> GMSDVAETLDPLRLPLQGERLIEASAGTGKTFTIAALYLRLLLGLGGSAAFPRPLTVEELLVVTFTEAATAELRGRIRSNIHELRIACLRETTDNPLYERLLEEIDDKAQAAQWLLLAERQMDEAAVFTIHGFCQRMLNLNAFESGMLFEQQLIEDESLLRYQACADFWRRHCYPLPREIAQVVFETWKGPQALLRDINRYLQGEAPVIKAPPPDDETLASRHAQIVARIDTVKQQWRDAVGELDALIESSGIDRRKFNRSNQAKWIDKISAWAEEETNSYQLPESLEKFSQRFLEDRTKAGGETPRHPLFEAIDQLLAEPLSIRDLVITRALAEIRETVAREKRRRGELGFDDMLSRLDSALRSESGEVLAAAIRTRFPVAMIDEFQDTDPQQYRIFRRIWHHQPETALLLIGDPKQAIYAFRGADIFTYMKARSEVHAHYTLDTNWRSAPGMVNSVNKLFSQTDDAFMFREIPFIPVKSAGKNQALRFVFKGETQPAMKMWLMEGESCGVGDYQSTMAQVCAAQIRDWLQAGQRGEALLMNGDDARPVRASDISVLVRSRQEAAQVRDALTLLEIPSVYLSNRDSVFETLEAQEMLWLLQAVMTPERENTLRSALATSMMGLNALDIETLNNDEHAWDVVVEEFDGYRQIWRKRGVMPMLRALMSARNIAENLLATAGGERRLTDILHISELLQEAGTQLESEHALVRWLSQHILEPDSNASSQQMRLESDKHLVQIVTIHKSKGLEYPLVWLPFITNFRVQEQAFYHDRHSFEAVLDLNAAPESVDLAEAERLAEDLRLLYVALTRSVWHCSLGVAPLVRRRGDKKGDTDVHQSALGRLLQKGEPQDAAGLRTCIEALCDDDIAWQTAQTGDNQPWQVNDVSTAELNAKTLQRLPGDNWRVTSYSGLQQRXXXXXXXXXXXXXXXXXXXXXXXXXPTLTPHQFPRGASPGTFLHSLFEDLDFTQPVDPNWVREKLELGGFESQWEPVLTEWITAVLQAPLNETGVSLSQLSARNKQVEMEFYLPISEPLIASQLDTLIRQFDPLSAGCPPLEFMQVRGMLKGFIDLVFRHEGRYYLLAYKSNWLGEDSSAYTQQAMAAAMQAHRYDLQYQLYTLALHRYLRHRIADYDYEHHFGGVIYLFLRGVDKEHPQQGIYTTRPNAGLIALMDEMFAGMTLEEA;> MLRVYHSNRLDVLEALMEFIVERERLDDPFEPEMILVQSTGMAQWLQMTLSQKFGIAANIDFPLPASFIWDMFVRVLPEIPKESAFNKQSMSWKLMTLLPQLLEREDFTLLRHYLTDDSDKRKLFQLSSKAADLFDQYLVYRPDWLAQWETGHLVEGLGEAQAWQAPLWKALVEYTHQLGQPRWHRANLYQRFIETLESATTCPPGLPSRVFICGISALPPVYLQALQALGKHIEIHLLFTNPCRYYWGDIKDPAYLAKLLTRQRRHSFEDRELPLFRDSENAGQLFNSDGEQDVGNPLLASWGKLGRDYIYLLSDLESSQELDAFVDVTPDNLLHNIQSDILELENRAVAGVNIEEFSRSDNKRPLDPLDSSITFHVCHSPQREVEVLHDRLLAMLEEDPTLTPRDIIVMVADIDSYSPFIQAVFGSAPADRYLPYAISDRRARQSHPVLEAFISLLSLPDSRFVSEDVLALLDVPVLAARFDITEEGLRYLRQWVNESGIRWGIDDDNVRELELPATGQHTWRFGLTRMLLGYAMESAQGEWQSVLPYDESSGLIAELVGHLASLLMQLNIWRRGLAQERPLEEWLPVCRDMLNAFFLPDAETEAAMTLIEQQWQAIIAEGLGAQYGDAVPLSLLRDELAQRLDQERISQRFLAGPVNICTLMPMRSIPFKVVCLLGMNDGVYPRQLAPLGFDLMSQKPKRGDRSRRDDDRYLFLEALISAQQKLYISYIGRSIQDNSERFPSVLVQELIDYIGQSHYLPGDEALNCDESEARVKAHLTCLHTRMPFDPQNYQPGERQSYAREWLPAASQAGKAHSEFVQPLPFTLPETVPLETLQRFWAHPVRAFFQMRLQVNFRTEDSEIPDTEPFILEGLSRYQINQQLLNALVEQDDAERLFRRFRAAGDLPYGAFGEIFWETQCQEMQQLADRVIACRQPGQSMEIDLACNGVQITGWLPQVQPDGLLRWRPSLLSVAQGMQLWLEHLVYCASGGNGESRLFLRKDGEWRFPPLAAEQALHYLSQLIEGYREGMSAPLLVLPESGGAWLKTCYDAQNDAMLDDDSTLQKARTKFLQAYEGNMMVRGEGDDIWYQRLWRQLTPETMEAIVEQSQRFLLPLFRFNQS;> MGKLQKQLLEAVEHKQLRPLDVQFALTVAGDEHPAVTLAAALLSHDAGEGHVCLPLSRLENNEASHPLLATCVSEIGELQNWEECLLASQAVSRGDEPTPMILCGDRLYLNRMWCNERTVARFFNEVNHAIEVDEALLAQTLDKLFPVSDEINWQKVAAAVALTRRISVISGGPGTGKTTTVAKLLAALIQMADGERCRIRLAAPTGKAAARLTESLGKALRQLPLTDEQKKRIPEDASTLHRLLGAQPGSQRLRHHAGNPLHLDVLVVDEASMIDLPMMSRLIDALPDHARVIFLGDRDQLASVEAGAVLGDICAYANAGFTAERARQLSRLTGTHVPAGTGTEAASLRDSLCLLQKSYRFGSDSGIGQLAAAINRGDKTAVKTVFQQDFTDIEKRLLQSGEDYIAMLEEALAGYGRYLDLLQARAEPDLIIQAFNEYQLLCALREGPFGVAGLNERIEQFMQQKRKIHRHPHSRWYEGRPVMIARNDSALGLFNGDIGIALDRGQGTRVWFAMPDGNIKSVQPSRLPEHETTWAMTVHKSQGSEFDHAALILPSQRTPVVTRELVYTAVTRARRRLSLYADERILSAAIATRTERRSGLAALFSSRE

The RecBCD/AddAB complexes are highly processive helicase/nuclease machines that digest DNA from the broken end until they encounter a crossover hotspot instigator (Chi) sequence. At this point their activities are modulated to produce a 3-tailed duplex onto which RecA is loaded. However, it was shown instead that the nuclease domain is actually a C-terminal domain of the RecB subunit, the activity of which is regulated by RecD. Consequently, RecBCD has evolved regulatory mechanisms that suppress activity unless the enzyme complex is bound to a bona fide DNA substrate (i.e. a broken DNA end).

In order to understand how the RecD subunit is able to activate the nuclease domain of RecB, we have now determined the cryo-electron microscopy (cryoEM) structure of RecBCD bound to a forked DNA substrate with an extended 5’-tail that spans the entire RecD subunit. We utilised a DNA fork substrate with a 25 base pair duplex region, capped at one end with a five base hairpin and at the other with unpaired 3’ and 5’-tails (3 and 12 thymidine residues, respectively). Electron density for bound ADPNP is visible in the ATP-binding site of the RecB subunit. Electron density corresponding to all twelve bases of the 5’-tail could be traced from the fork junction, across and through the RecC subunit, and along a groove on the RecD subunit. In previous structures of RecBCD, the RecD subunit adopted an open conformation but in the current structure the protein closes around and clamps the 5’ ssDNA tail. The closing of the RecD clamp brings the SH3 domain of RecD into contact with the 2B domain of the RecB subunit that appears to act as a catch to stabilise the closed conformation of RecD. The 2B domain of the RecD subunit is visible in our current EM structure and confirms the fold of this domain is similar to that of the SH3 fold observed for RecD2. First, several domains of the RecC subunit also undergo a change in conformation. In the initiation complex, the α-helix that blocks the nuclease active site is stabilised by stacking contacts with another α-helix (residues 602–627) from the 2B domain of RecC. This interaction is altered as a consequence of the conformational changes in the RecC subunit that shift the position of the RecC helix, breaking the contacts with the nuclease-blocking helix of the RecB linker, resulting in release of this helix from the nuclease active site, for which there is now no electron density.> 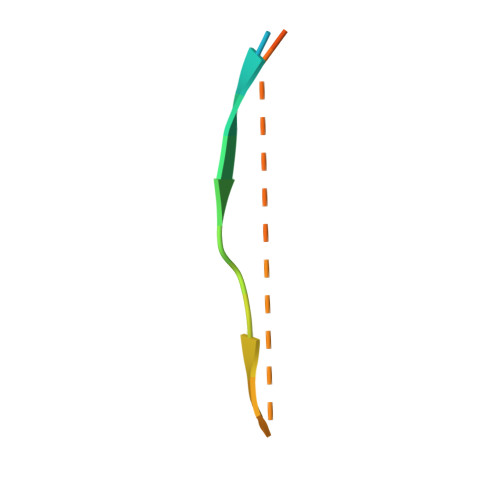GSGPQAQIAKPIRSGQGATS>SISSRVKSKRIQLGLNQAELAQKVGTTQQSIEQLENGKTKRPRFLPELASAL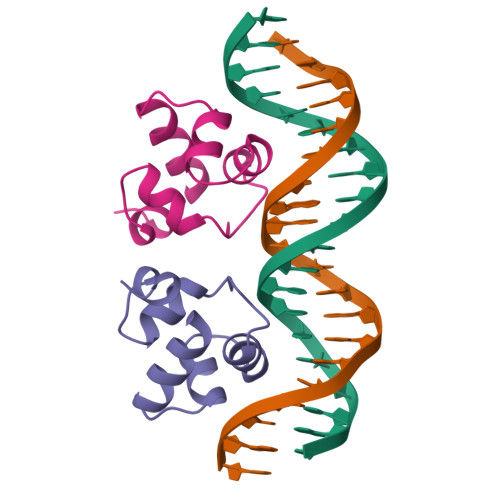GVSVDWLLNGTSDSNVR[2x]>NAQFLHTQVGRGLLGAVVNPLGEVTDKFAVTDNSEILYRPVDNAPPLYSERAAIEKPFLTGIKVIDSLLTCGEGQRMGIFASAGCGKTFLMNMLIEHSGADIYVIGLIGERGREVTETVDYLKNSEKKSRCVLVYATSDYSSV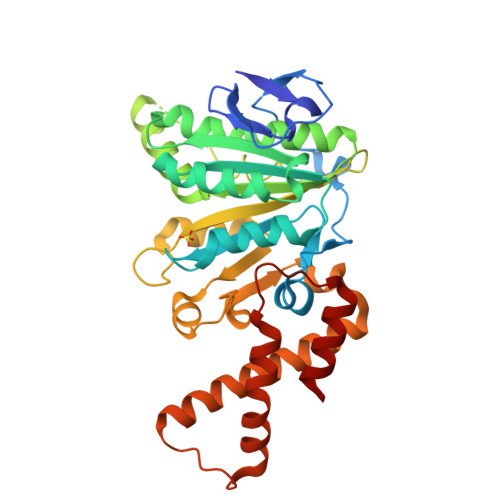DRCNAAYIATAIAEFFRTEGHKVALFIDSLTRYARALRDVALAAGESPAERGYPVSVFDSLPRLLERPGKLKAGGSITAFYTVLLEDDDFADPLAEEVRSILDGHIYLSRNLAQKGQFPAIDSLKSISRVFTQVVDEKHRIMAAAFRELLSEIEELRTIIDFGEYKPGENASQDKIYNKISVVESFLKQDYRLGFTYEQTMELIGETIR[2x]> GSMSESADLTELYSIIEKTAQVVDVTASHDKVWPILNAFQDVIADSVISFRASTGSSADDLDCRFTMLPKGLDPYARALEHGLTPKTDHPVGSLLKEVHENLPITSCGVDFGVAGGFTKTWSFPSAEKLGKVSELVKLPSIPDAVAANRDFFEKWGIADMVSTVGIDYSKRTMNLYFGGGVGDRVPAGVFEEKGVRAILGELGLAAPSEELLKFCERSFVIYVTLSWDSPKINRFTYSVMTPEPLGLPVDLAPTFERLIKSAPYDTEGRNYVYGIASTPKGEYHKIASYYQWQKRVEKLLRSDG

The PT EpzP from Streptomyces cinnamonensis DSM 1042 reported here is a member of a new type of bacterial prenyltransferases, as it catalysis the prenylation of a phenazine substrate. EpzP is a soluble, monomeric ABBA PT consisting of 302 amino acids with a molecular mass of 33.2 kDa. The overall structure of EpzP belongs to the PT-fold family and is characterized by ten antiparallel β-strands that assemble into a circular β-barrel. The β-barrel houses a solvent-filled reaction chamber in which the substrates bind and the regioselective Friedel-Crafts prenylation of dhPCA takes place.

Structure analysis of this crystal from (EpzPwt) and comparison with the two earlier structures confirmed that lysine methylation had not led to structural changes in the protein. Moreover, the EpzPwt structure showed that, in contrast to EpzPm-SPP and EpzPm-nat, the C-terminal portion of the enzyme was visible in the electron density and found to seal one entrance of the β-barrel. One of these, the C-terminal 310-helix in EpzPwt, seals the reaction chamber of the aromatic binding site of dhPCA. The aromatic binding pocket of dhPCA is located opposite to the diphosphate binding site, within a large cavity inside EpzPwt. Interestingly, we found substantial electron density in the cavity of EpzPwt, in an area near the predicted binding site of dhPCA. The density is indicative of the presence of an ordered compound. Although we were not able to unambiguously identify the nature of this compound, we conclude that it is inserted into the enzyme during protein production, as the shape of the density does not fit with any molecules used in downstream purification and crystallization experiments. In the closed structure of EpzPwt, R267 points towards the active center, whereas in the opened structure of EpzPm-SPP R267 is orientated to the solvent. The aromatic substrate dhPCA was docked in silico into the active site of EpzPwt by the use of Vina. However, as crystals of EpzPwt were not reproducible and other crystal forms could not be obtained, we were unable to prepare a ternary complex.> GPLGSMERKISRIHLVSEPSITHFLQVSWEKTLESGFVITLTDGHSAWTGTVSESEISQEADDMAMEKGKYVGELRKALLSGAGPADVYTFNFSKESCYFFFEKNLKDVSFRLGSFNLEKVENPAEVIRELICYCLDTIA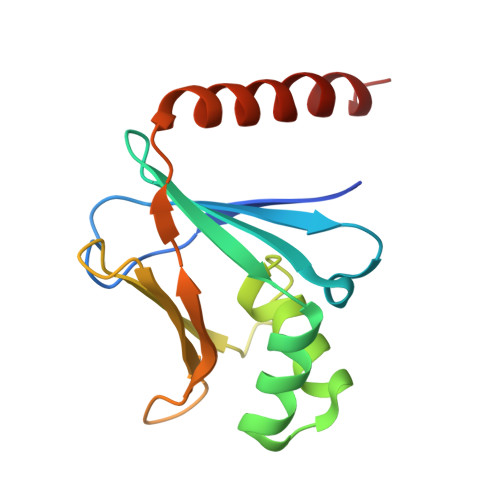ENQAK>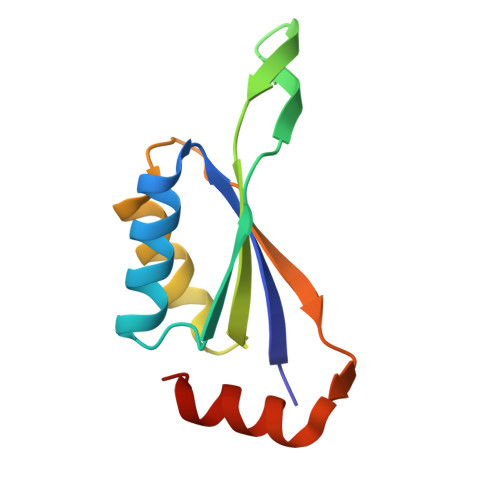 GGEEVVLITVPSALVAVKIAHALVEERLAACVNIVPGLTSIYREEGSVVSDHELLLLVKTTTDAFPKLKERVKELHPYEVPEIVALPIAEGNREYLDWLRENTGLE> GACGCGACCGAAUGAAAUGGUGAAGGACGGGUCCAGCCGGCUGC;> GCAGCCGGCU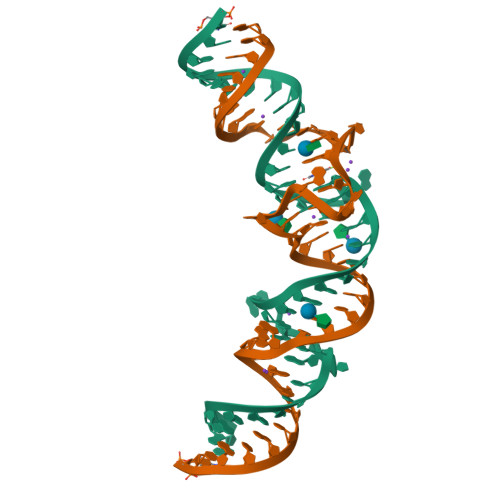UGUUGAGUAGAGUGUGAGCUCCGUAACUGGUCGCGUC>[4x]IVGGYTCEENSLPYQVSLNSGSHFCGGSLISEQWVVSAAHCYKTRIQVRLGEHNIKVLEGNEQFINAAKIIRHPKYNRDTLDNDIMLIKLSSPAVINARVSTISLPTAPPAAGTECLISGWGNTLSFGADYPDELKCLDAPVLTQAECKASYPGKITNSMFCVGFLEGGKDSC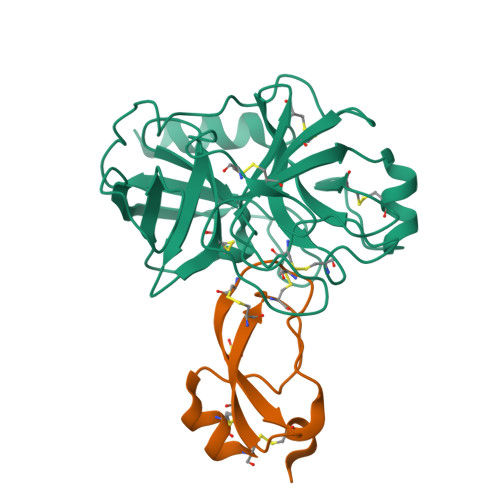QRDAGGPVVCNGQLQGVVSWGHGCAWKNRPGVYTKVYNYVDWIKDTIAANS;>YVDYKDDDDKEFMHSFCAFKADDGPCRACMKRFFFNIFTRQCEEFCYGGCEGNQNRFESLEECKKMCTRDPRHHHHHHAN[4x]> MRACLKCK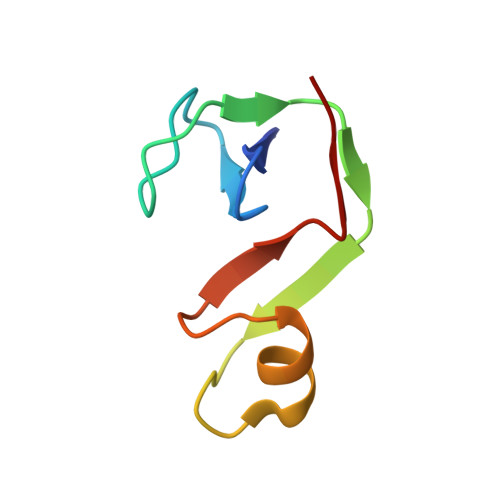YLTNDEICPICHSPTSENWIGLLIVINPEKSEIAKKAGIDIKGKYALSVKE> MSPILGYWKIKGLVQPTRLLLEYLEEKYEEHLYERDEGDKWRNKKFELGKHGHGHGKHKNKGLEFPNLPYYIDGDVKLTQSMAIIRYIADKHNMLGGCPKERAEISML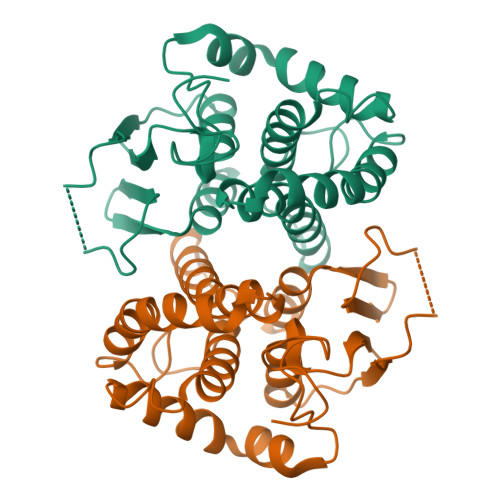EGAVLDIRYGVSRIAYSKDFETLKVDFLSKLPEMLKMFEDRLCHKTYLNGDHVTHPDFMLYDALDVVLYMDPMCLDAFPKLVCFKKRIEAIPQIDKYLKSSKYIAWPLQGWQATFGGGDHPPK>MAEEIKKQVQVNVDDIRAANIKLDGLGRQIADISNSISTIESRLGEMDNRLVGISSQVTQLSNSVSQ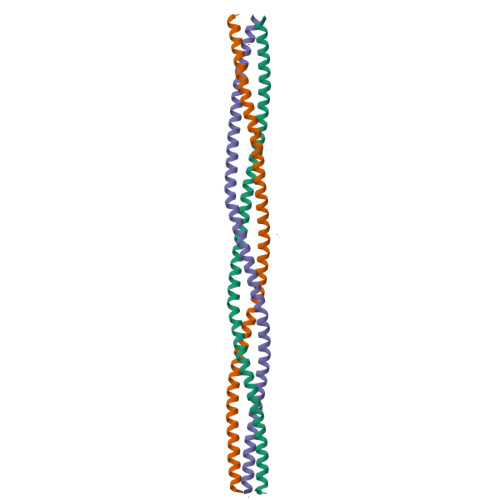NTQSISSLGDRINAVEPRVDSLDTVTSNLTGRTSTLEADVGSLRTELAALTTRVTTEVTRLDGLIN[3x]> PSTT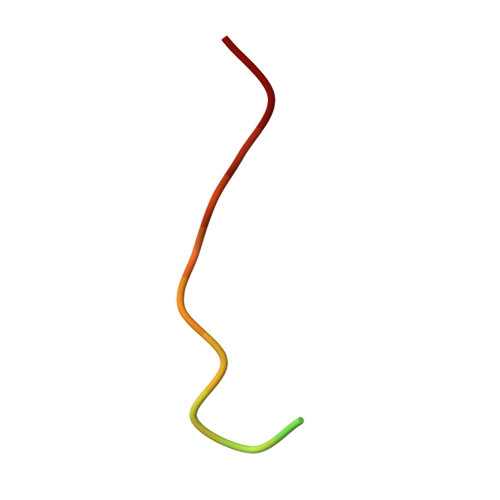KSFKNAPLLAPP> MAEYKDNLLGEANSFLEVLEQVSHLAPLDKPVLIIGERGTGKELIASRLHYLSSRWQGPFISLNCAALNENLLDSELFGHEAGAFTG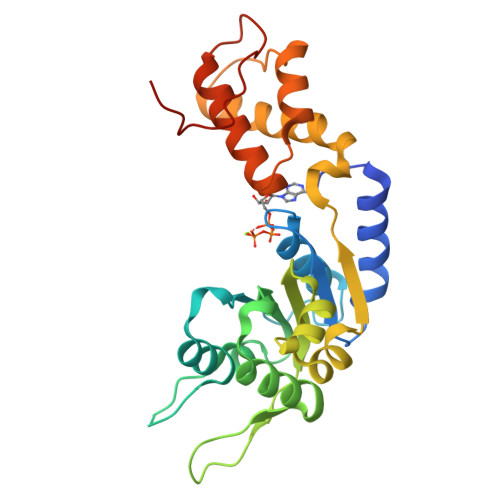AQKRHPGRFERADGGTLFLDELATAPMMVQEKLLRVIEYGELERVGGSQPLQVNVRLVCATNADLPAMVNEGTFRADLLDRLAFDVVQLPPLRERESDIMLMAEYFAIQMCREIKLPLFPGFTERARETLLNYRWPGNIAELKNVVERSVYRHGTSDYPLDDIIIDPFKRRPPEDAIA>MANPTLFVSYDQNGKKLSFANWISVLSPQDTPFVSMTGKESINQTIFSWQTDALASVDGNNAHVEGSRAEDGEMKPTVIKSNVTQILRKVVRVSDTANTTANYGRGRELMYQLEKKGKEIKRDLEKILLSGQARTDVLADQYLTNSAADPAVAGLNDTHAARKTGAFQFLCAHGGLAGGVVDKTKNGPADPDTGAVTVKVAQNASNPTTNIGFDEADIFDMTLQLYTAGSEADIIMINPAHAKIFAGLQENTQGSRKRIFENTKQFIYEVNSITDPLGQSYKIIVNRWMPTDAVY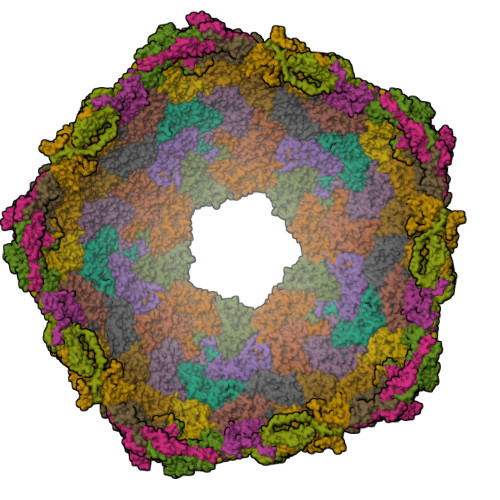FFRSADWTQMVLRAPKRTELAKDGSYEKWMIEMEVGLRHRNPYASGVLFTAAGKAAA[17x]>AVAITREEFLQGLLQSSRDFVARGKLKAPKWPILKNLELLQAQNYSRNIKTFPYKELNKSMYYDKWVCMCRCEDGALHFTQLKDSKTITTITTPNPRTGGEHPAIISRGPCNRLLLLYPGNQITILDSKTNKVLREIEVDSANEIIYMYGHNEVNTEYFIWADNRGTIGFQSYEDDSQYIVHSAKSDVEYSSGVLHKDSLLLALYSPDGILDVYNLSSPDQASSRFPVDEEAKIKEVKFADNGYWMVVECDQTVVCFDLRKDVGTLAYPTYTIPEFKTGTVTYDIDDSGKNMIAYSNESNSLTIYKFDKKTKNWTKDEESALCLQSDTADFTDMDVVCGDGGIAAILKT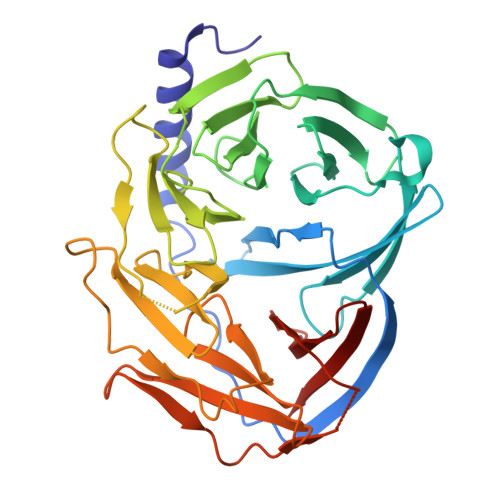NDSFNIVALTP[2x]> KEFTLDFSTAKTYVDSLNVIRSAIGTPLQTISSGGTSLLMIDSGTGDNLFAVDVRGIDPEEGRFNNLRLIVERNNLYVTGFVNRTNNVFYRFADFSHVTFPGTTAVTLSGDSSYTTLQRVAGISRTGMQINRHSLTTSYLDLMSHSGTSLTQSVARAMLRFVTVTAEALRFRQIQRGFRTTLDDLSGRSYVMT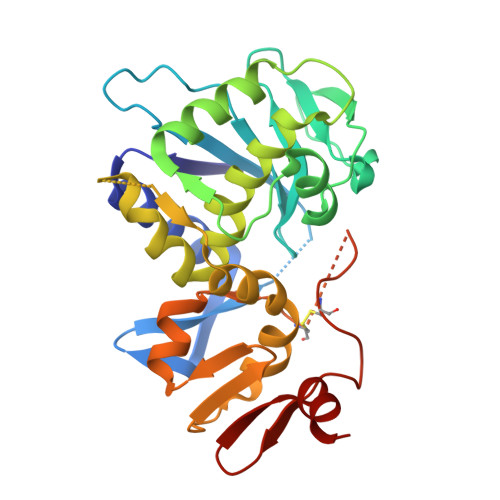AEDVDLTLNWGRLSSVLPDYHGQDSVRVGRISFGSINAILGSVALILNCHHHASRVARMASDEFPSMCPADGRVRGITHNKILWDSSTLGAILM>MAQNDNYIYSTEVGGVGGTPFTFMQESGTITSIKFNWSDQYKLLHHIEVKFINNANIYATGDPKGNHEVILEID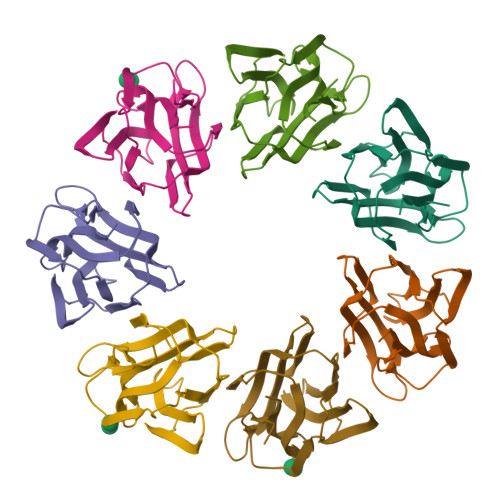DDETIIGSVIGYKKGNDGRCTGVKLTTSKGKSIMAGYFEESLITTYTGKLAGIKGGAGSDIDRLGLIFLKK[14x]>[2x]NYPAEPFRIKSVETVSMIPRDERLKKMQEAGYNTFLLNSKDIYIDLLTDSGTNAMSDKQWAGMMMGDEAYAGSENFYHLERTVQELFGFKHIVPTHQGRGAENLLSQLAIKPGQYVAGNMYFTTTRYHQEKNGAVFVDIVRDEAHDAGLNIAFKGDIDLKKLQKLIDEKGA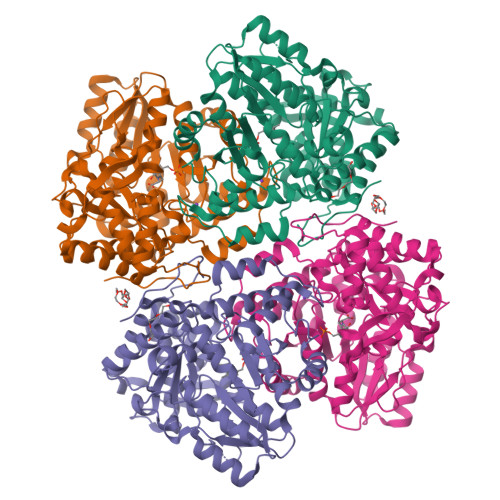ENIAYICLAVTVNLAGGQPVSMANMRAVRELTAAHGIKVFYDATRCVENAYFIKEQEQGFENKSIAEIVHEMFSYADGCTMSGKKDCLVNIGGFLCMNDDEMFSSAKELVVVYEGMPSYGGLAGRDMEAMAIGLREAMQYEYIEHRVKQVRYLGDKLKAAGVPIVEPVGGHAVFLDARRFCEHLTQDEFPAQSLAASIYVETGVRSMERGIISAGRNNVTGEHHRPKLETVRLTIPRRVYTYAHMDVVADGIIKLYQHKEDIRGLKFIYEPKQLRFFTARFDYI Centromeric chromatin in fission yeast is distinguished by the presence of nucleosomes containing the histone H3 variant Cnp1CENP-A. Cell cycle–specific deposition of Cnp1 requires the Mis16–Mis18–Mis19 complex, which is thought to direct recruitment of Scm3-chaperoned Cnp1/histone H4 dimers to DNA. Mis16 is a homologue of the human WD40-repeat protein RbAp46/48, a well-known histone chaperone found in a variety of chromatin-associated complexes, whereas Mis19 seems to form a bridge between Mis16 and Mis18 with its N terminus binding Mis18 and C terminus binding Mis16. Current structural and biochemical data suggest a model in which Mis18 provides the principal link to the centromere, whereas Mis16 is responsible for recruitment of the Scm3–Cnp1–H4 complex, which allows Cnp1–H4 dimers to be inserted into chromatin as a prelude to complete nucleosome assembly. As expected, Mis16 adopts a β-propeller fold, consisting of 7 WD-40 repeats, with an extended N-terminal α-helix that forms part of the histone interaction pocket.

We first solved the crystal structure of S. pombe Mis16 both alone and with the N terminus (residues 14–44) of histone H4 bound at 1.9 and 1.8 Å resolution, respectively. Overall, the structure of S. pombe Mis16 and its interactions with histone H4 closely resemble those of the homologous Schizosaccharomyces japonicus Mis16 and the human RbAp46/48 proteins and exhibit a highly conserved interface, which has been extensively described by others. Residues 56–63 form a β-strand that continues β-propeller 7 of Mis16 and stabilises an extended loop from 107 to 116, which is disordered in the Mis16 structure alone.

> GSEEVVQDAPLENNELNAEIDLQKTIQEEYKLWKQNVPFLYDLVITHALEWPSLTIQWLPDKKTIPGTDYSIQRLILGTHTSGNDQNYLQIASVQLPNFDEDTTEFTPSTIRRAQATGSYTIEISQKIPHDGDVNRARYMPQKPEIIATMGEGGNAYIFDTTCHDALTTGEALPQAVLKGHTAEGFGLCWNPNLPGNLATGAEDQVICLWDVQTQSFTSSETKVISPIAKYHRHTDIVNDVQFHPQHEALLASVSDDCTLQIHDTRLNPEEEAPKVIQAHSKAINAVAINPFNDYLLATASADKTVALWDLRNPYQRLHTLEGHEDEVYGLEWSPHDEPILASSSTDRRVCIWDLEKIGEEQTPEDAEDGSPELLFMHGGHTNRISEFSWCPNERWVVGSLADDNILQIWSPSRVIWGRDHVQVSPRDLE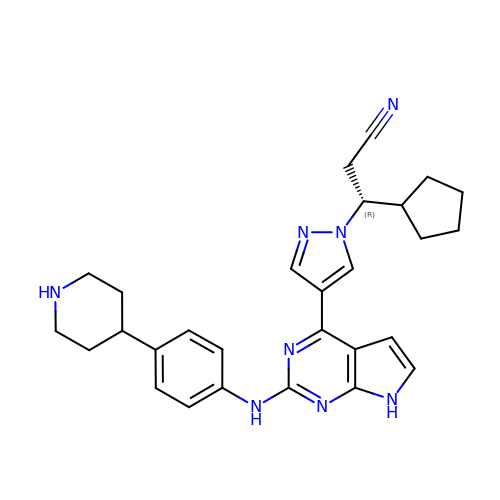(3R)-3-cyclopentyl-3-[4-(2-{[4-(piperidin-4-yl)phenyl]amino}-7H-pyrrolo[2,3-d]pyrimidin-4-yl)-1H-pyrazol-1-yl]propanenitrile | C28 H32 N8 | RGIJZWRVCBSGJV-RUZDIDTESA-N>MGSSHHHHHHSQDPMVLLHKSTHIFPTDFASVSRAFFNRYPNPYSPHVLSIDTISRNVDQEGNLRTTRLLKKSGKLPTWVKPFLRGITETWIIEVSVVNPANSTMKTYTRNLDHTGIMKVEEYTTYQFDSATSSTIADSRVKFSSGFNMGIKSKVEDWSRTKFDENVKKSRMGMAFVIQKLEEARNPQF[6x];>[6x]MGNIMSASFAPECTDLKTKYDSCFNEWYSEKFLKGKSVENECSKQWYAYTTCVNAALVKQGIKPALDEAREEAP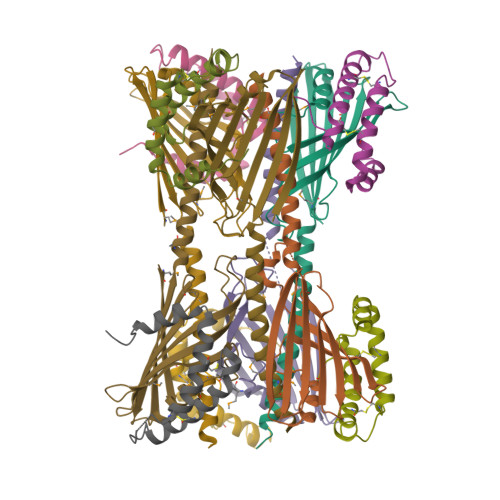FENGGKLKEVDK>[14x]GQMAYDRAITVFSPDGRLFQVEYAREAVKKGSTALGMKFANGVLLISDKKVRSRLIEQNSIEKIQLIDDYVAAVTSGLVADARVLVDFARISAQQEKVTYGSLVNIENLVKRVADQMQQYTQYGGVRPYGVSLIFAGIDQIGPRLFDCDPAGTINEYKATAIGSGKDAVVSFLEREYKENLPEKEAVTLGIKALKSSLEEGEELKAPEIASITVGNKYRIYDQEEVKKFL;>[14x]TTTVGITLKDAV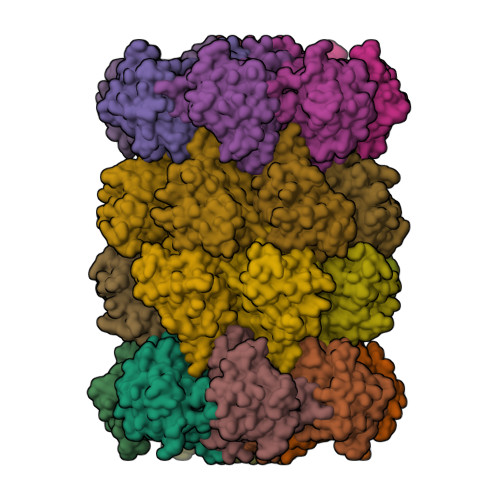IMATERRVTMENFIMHKNGKKLFQIDTYTGMTIAGLVGDAQVLVRYMKAELELYRLQRRVNMPIEAVATLLSNMLNQVKYMPYMVQLLVGGIDTAPHVFSIDAAGGSVEDIYASTGSGSPFVYGVLESQYSEKMTVDEGVDLVIRAISAAKQRDSASGGMIDVAVITRKDGYVQLPTDQIESRIRKLGLIL> LLFVQRDSK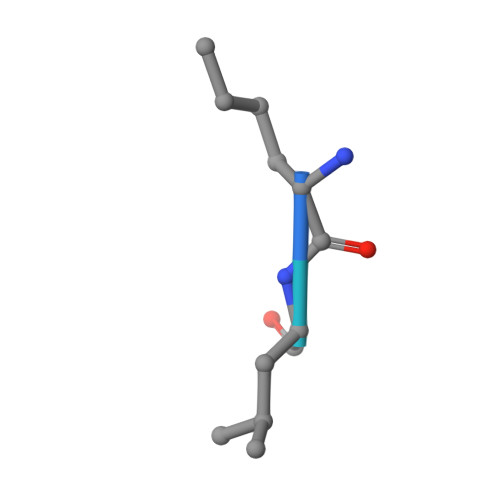E> MSAASSQHVLLSPAELAYLHASLSLTPPIRPDGRSPTQFRPLIAETGILPGANGSARVCFADGTEAIVGVKAEVEKTVSRSKEDEEVGLLVASAGDMDVDDEEGYAKVGADNRTGEASWVEITVEIPGVRDDDSGMVFLAQLLGEALLADGEFVKKLWINRRYHWKLYIDILLISPPLSYPLPLLSLTTHLALLSTRLPRLKSEGDEDPYFDDDWAVAPYLFPRSSSASKSSKSSPTQPTTRPPITLLVMAVGNNILFDPSKEELAVADVALAVSVTATDVDPDESDAQKETATATAGPDSADAAKRGRKLRLLSIRTIDPPSRLTPPGVPNSTNPAAIYGTTSSSGTNGNGQPQQKVESGKISEPIEPIEGVWRAPRGGAKRLVLGALVQKVLEKGGVVDEVLD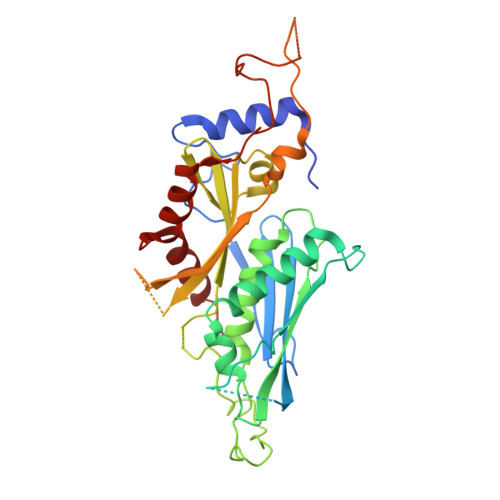ALEGVELT> SKGKSS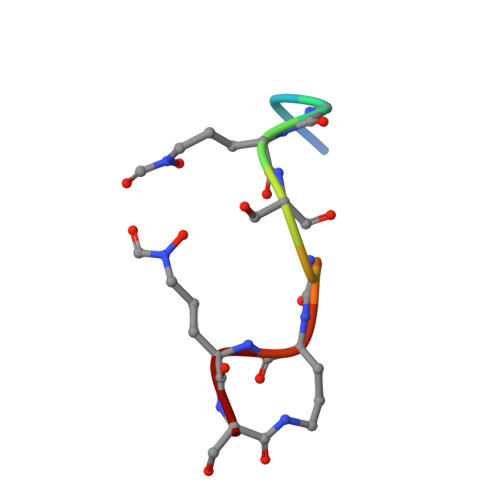GAKS> MKVVYDDVRVLKDIIQALARLVDEAVLKFKQDSVELVALDRAHISLISVNLPREMFKEYDVNDEFKFGFNTQYLM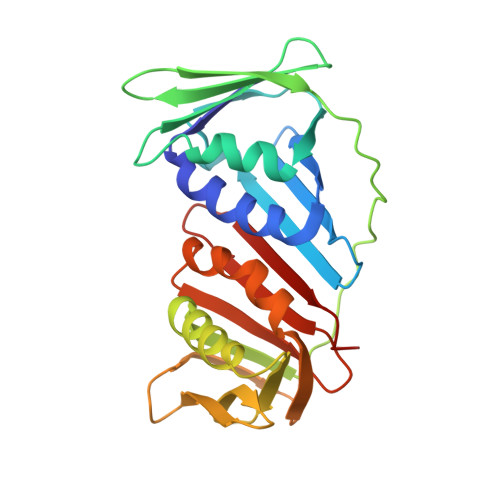KILKVAKRKEAIEIASESPDSVIINIIGSTNREFNVRNLEVSEQEIPEINLQFDISATISSDGFKSAISEVSTVTDNVVVEGHEDRILIKAEGESEVEVEFSKDTGGLQDLEFSKESKNSYSAEYLDDVLSLTKLSDYVKISFGNQKPLQLFFNMEGGGKVTYLLAPKV>MGSSHHHHHHSSGENLYFQGHMMPVALTIAGSDSGGGAGIQADLKTFSALGVYGMSVITAVTAQNTLGVQGVHDIPPELVAAQIDAVFEDLRVDAVKTGMLSNAEIVEAVAEALRRYGVRPLVVDPVMVAKSGDPLLAPDAVEALKERLFPLATIITPNLPEAEVLLGRPIRTEEEMEEAARRLLALGPKAVLLKGGHLEGEEAVDLLADGEGIHRFSAPRVQTRNTHGTGCTLSAAIAAHLARGHDLPE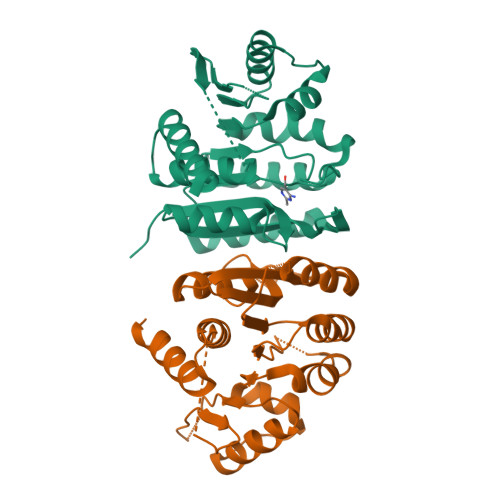AVREAKAYLTGAIKAAPSIGHGHGPVNHFHAWWKRAE[2x]> MPVITVNTNVAEKSIPVFFQAALTNMMTKALQKPKEVMFVDLRSGANIMMGGDRNPCVFATVECIGRLNPTSNLAMARDMEDMFIEHLNVRRERIVIRFIP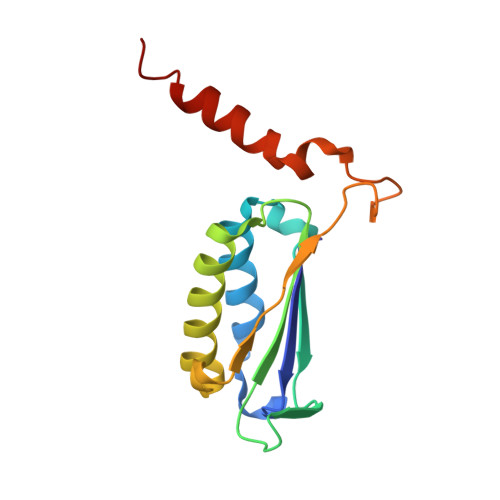VPALFCSFNGALHDVSIERDEDIISQAIAEAAHHHA> MHHHHHHMNFNVSLMEKLKWKIKCIENKFLNYRLTTNETVVAETEYGKVKGVKRLTVYDDSYYSFEGIP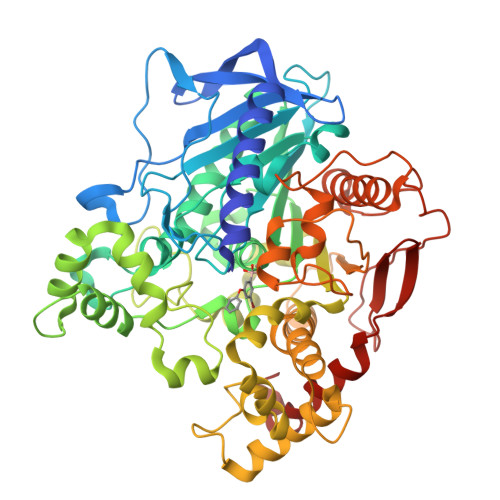YAQPPVGELRFKAPQRPTPWAGVRDCCNHKDKSVQVDFITGKVCGSEDCLYLSVYTNNLNPETKRPVLVYIHGGDFIIGENHRDMYGPDYFIKKDVVLINIQYRLGALGFLSLNSEDLNVPGNAGLKDQVMALRWIKNNCANFGGNPDNITVFGESAGAASTHYMMLTEQTRGLFHRGILMSGNAICPWANTQCQHRAFTLAKLAGYKGEDNDKDVLEFLMKAKPQDLIKLEEKVLTLEERTNKVMFPFGPTVEPYQTADCVLPKHPREMVKTAWGNSIPTMMGNTSYEGLFFTSILKQMPLLVKELETCVNFVPSELADAERTAPETLEMGAKIKKAHVTGETPTADNFMDLCSHFYFWFPMHRLLQLRFNHTSGTPVYLYRFDFDSEDLINPYRIMRSGRGVKGVSHTDELTYFFWNQLAKRMPKESREYKTIERMTGIWTQFATTGNPYSNEIEGMENVSWDPIEKSDEVYKCLNISDELKMIDVPEMGKIKQWESMFEKHRDLF>[2x]MRVPEKYSTLPAEDRSVHIVNICAIEDLGYLPSEGTLLNSLSVDPDAECKYGLYFRDGKRKVDYILVYHHKRASGSRTLARRGLQNDMVLGTRSVRQDQPLPGKGSPVDAGSPEVPMDYHEDDKRFRREEYEGNLLEAGLELENDEDTKIHGVGFVKIHAPWHVLCREAEFLKLKMPTKKVYHISETRGLLKTINSVLQKITDPIQPKVAEHRPQTTKRLSYPFSREKQHLFDLTDRDSFFDSKTRSTIVYEILKRTTCTKAKYSMGITSLLANGVYSAAYPLHDGDYEGDNVEFNDRKLLYEEWASYGVFYKYQPIDLVRKYFGEKVGLYFAWLGAYTQMLIPASIVGVIVFLYGCATVDENIPSMEMCDQRYNITMCPLCDKTCSYWKMSSACATARASHLFDNPATVFFSVFMALWAATFMEHWKRKQMRLNYRWDLTGFEEEEEAVKDHPRAEYEARVLEKSLRKESRNKETDKVKLTWRDRFPAYFTNLVSIIF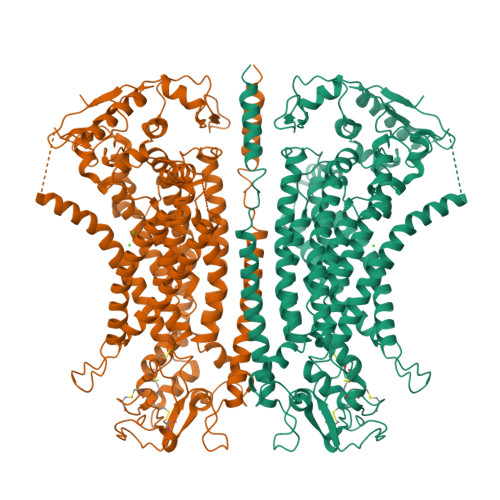MIAVTFAIVLGVIIYRISTAAALAMNSSPSVRSNIRVTVTATAVIINLVVIALLDEVYGCIARWLTKIEVPKTEKSFEERLTFKAFLLKFVNSYTPIFYVAFFKGRFVGRPGDYVYIFRSFRMEECAPGGCLMELCIQLSIIMLGKQLIQNNLFEIGIPKMKKFIRYLKLRRQSPSDREEYVKRKQRYEVDFNLEPFAGLTPEYMEMIIQFGFVTLFVASFPLAPLFALLNNIIEIRLDAKKFVTELRRPVAIRAKDIGIWYNILRGVGKLAVIINAFVISFTSDFIPRLVYLYMYSQNGTMHGFVNHTLSSFNVSDFQNGTAPNDPLDLGYEVQICRYKDYREPPWSEHKYDISKDFWAVLAARLAFVIVFQNLVMFMSDFVDWVIPDIPKDISQQIHKEKVLMVELFMREEQGKQQLLDTWMEKEKPRDVPCNNHSPTTHPEAGDGSPVPSYEYHGDAL>HHHHHHFNLPPGNYKKPKLLYCSNGGHFLRILPDGTVDGTRDRSDQHIQLQLSAESVGEVYIKSTETGQYLAMDTDGLLYGSQTPNSNCLFLERLEENHYNTYISKAHAEKNWFVGLKKNGSCKRGPRTHYGQKAILFLPLPVSSD[2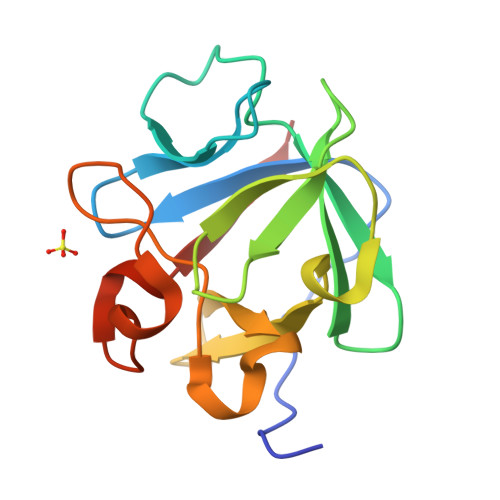x]>MHHHHHHAAGIPMNNPAIKRIGNHITKSPEDKREYRGLELANGIKVLLISDPTTDKSSAALDVHIGSLSDPPNIAGLSHFCQHMLFLGTKKYPKENEYSQFLSEHAGSSNAFTSGEHTNYYFDVSHEHLEGALDRFAQFFLCPLFDESCKDREVNAVDSEHEKNVMNDAWRLFQLEKATGNPKHPFSKFGTGNKYTLETRPNQEGIDVRQELLKFHSAYYSSNLMAVCVLGRESLDDLTNLVVKLFSEVENKNVPLPEFPEHPFQEEHLKQLYKIVPIKDIRNLYVTFPIPDLQKYYKSNPGHYLGHLIGHEGPGSLLSELKSKGWVNTLVGGQKEGARGFMFFIINVDLTEEGLLHVEDIILHMFQYIQKLRAEGPQEWVFQECKDLNAVAFRFKDKERPRGYTSKIAGILHYYPLEEVLTAEYLLEEFRPDLIEMVLDKLRPENVRVAIVSKSFEGKTDRTEEWYGTQYKQEAIPDEVIKKWQNADLNGKFKLPTKNEFIPTNFEILPLEKEATPYPALIKDTAMSKLWFKQDDKFFLPKACLNFEFFSPFAYVDPLHCNMAYLYLELLKDSLNEYAYAAELAGLSYDLQNTIYGMYLSVKGYNDKQPILLKKIIEKMATFEIDEKRFEIIKEAYMRSLNNFRAEQPHQHAMYYLRLLMTEVAWTKDELKEALDDVTLPRLKAFIPQLLSRLHIEALLHGNITKQAALGIMQMVEDTLIEHAHTKPLLPSQLVRYREVQLPDRGWFVYQQRNEVHNNCGIEIYYQTDMQSTSENMFLELFCQIISEPCFNTLRTKEQLGYIVFSGPRRANGIQGLRFIIQSEKPPHYLESRVEAFLITMEKSIEDMTEEAFQKHIQALAIRRLDKPKKLSAECAKY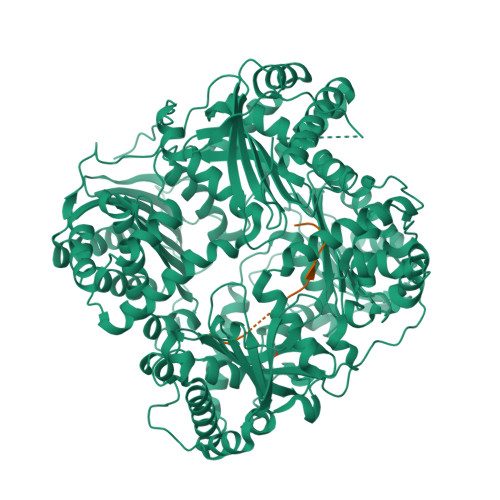WGEIISQQYNFDRDNTEVAYLKTLTKEDIIKFYKEMLAVDAPRRHKVSVHVLAREMDSCPVVGEFPCQNDINLSQAPALPQPEVIQNMTEFKRGLPLFPLVKPHINFMAAKL[2x];>[2x]AAAAAAAAAAAA>MASKLLRAVILGPPGSGKGTVCQRIAQNFGLQHLSSGHFLRENIKASTEVGEMAKQYIEKSLLVPDHVITRLMMSELENRRGQHWLLDGFPRTLGQAEALDKICEVDLVISLNIPFETLKDRLSRRWIHPPSGRVYNLDFNPPHVHGIDDVTGE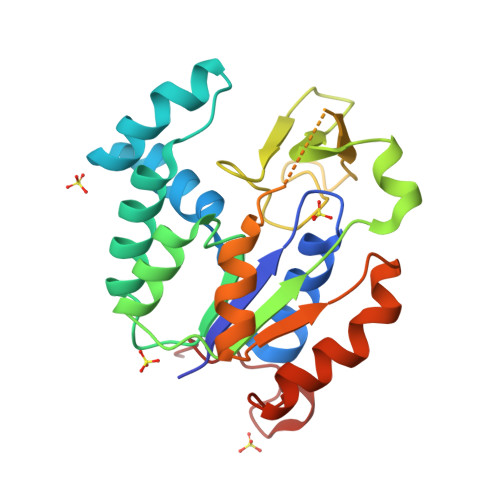PLVQQEDDKPEAVAARPRQYKDVAKPVIELYKSRGVLHQFSGTETNKIWPYVYTLFSNKITPIQSKEAYLEHHHHHH[2x]> MAAAAPNAGGSAPETAGSAEAPLQYSLLLQYLVGDKRQPRLLEPGSLGGIPSPAKSEEQKMIEKAMESCAFKAALACVGGFVLGGAFGVFTAGIDTNVGFDPKDPYRTPTAKEVLKDMGQRGMSYAKNFAIVGAMFSCTECLIESYRGTSDWKNSVISGCITGGAIGFRAGLKAGAIGCGGFAAFSAAIDYYLR;> MTVFFKTLRNHWKKTTAGLCLLTWGGHWLYGKHCDNLLRRAACQEAQVFGNQLIPPNAQVKKATVFLNPAACKGKARTLFEKNAAPILHLSGMDVTIVKTDYEGQAKKLLELMENTDVIIVAGGDGTLQEVVTGV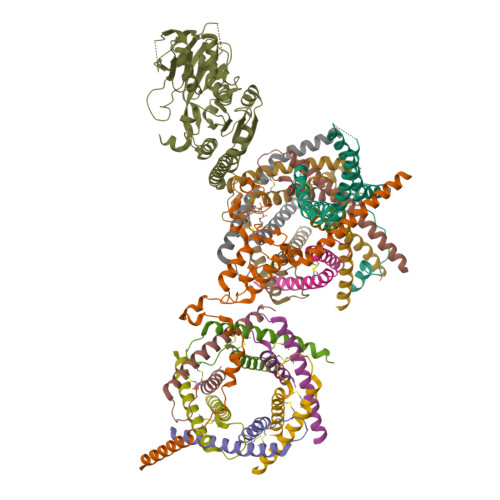LRRTDEATFSKIPIGFIPLGETSSLSHTLFAESGNKVQHITDATLAIVKGETVPLDVLQIKGEKEQPVFAMTGLRWGSFRDAGVKVSKYWYLGPLKIKAAHFFSTLKEWPQTHQASISYTGPTERPPNEPEETPVQRPSLYRRILRRLASYWAQPQDALSQEVSPEVWKDVQLSTIELSITTRNNQLDPTSKEDFLNICIEPDTISKGDFITIGSRKVRNPKLHVEGTECLQASQCTLLIPEGAGGSFSIDSEEYEAMPVEVKLLPRKLQFFCDPRKREQMLTSPTQ;> MAAAALRRFWSRRRAEAGDAVVAKPGVWARLGSWARALLRDYAEACRDASAEARARPGRAAVYVGLLGGAAACFTLAPSEGAFEEALLEASGTLLLLAPATRNRESEAFVQRLLWLRGRGRLRYVNLGLCSLVYEAPFDAQASLYQARCRYLQPRWTDFPGRVLDVGFVGRWWVLGAWMRDCDINDDEFLHLPAHLRVVGPQQLHSETNERLFDEKYKPVVLTDDQVDQALWEEQVLQKEKKDRLALSQAHSLVQAEAPR;>[5x]MAAQIPESDQIKQFKEFLGTYNKLTETCFLDCVKDFTTREVKPEETTCSEHCLQKYLKMTQRISMRFQEYHIQQNEALAAKAGLLGQPR;>[6x]MDPLRAQQLAAELEVEMMADMYNRMTSACHRKCVPPHYKEAELSKGESVCLDRCVSKYLDIHERMGKKLTELSMQDEELMKRVQQSSGPA;> MERQQQQQQQLRNLRDFLLVYNRMTELCFQRCVPSLHHRALDAEEEACLHSCAGKLIHSNHRLMAAYVQLMPALVQRRIADYEAASAVPGVAAEQPGVSPSGS(3R,4R)-1-METHANESULFONYL-PYRROLIDINE-3,4-DICARBOXYLIC ACID 3-[(4-CHLORO-3-FLUORO-PHENYL)-AMIDE] 4-{[2-FLUORO-4-(2-OXO-2H-PYRIDIN-1-YL)-PHENYL]-AMIDE} 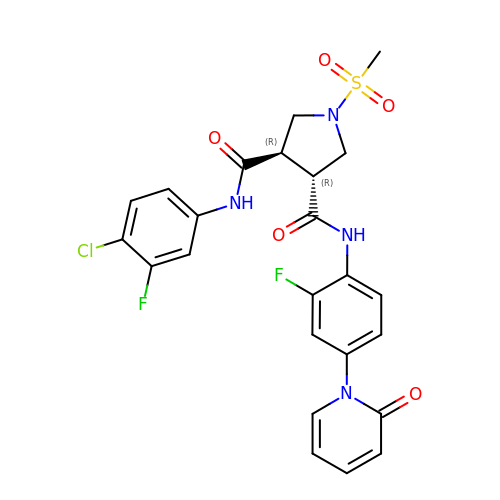| C24 H21 Cl F2 N4 O5 S | XRNMSDIWHHURFN-IRXDYDNUSA-N> SIPGQVADQAPLPSLAPMLEKVLPAVVSVRVEGTASQGQKIPEEFKKFFGDDLPDQPAQPFEGLGSGVIINASKGYVLTNNHVINQAQKISIQLNDGREFDAKLIGSDDQSDIALLQIQNPSKLTQIAIADSDKLRVGDFAVAVGNPFGLGQTATSGIVSALGRSGLNLEGLENFIQTDASINRGNSGGALLNLNGELIGINTAILAPGGGSVGIGFAIPSNMARTLAQQLIDFGEIKRGLLGIKGTEMSADIAKAFNLDVQRGAFVSEVLPGSGSAKAG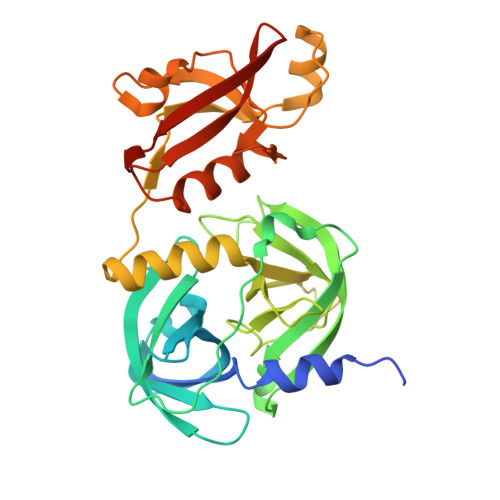VKAGDIITSLNGKPLNSFAELRSRIATTEPGTKVKLGLLRNGKPLEVEVTLDTSTSSLEHHHHHH The viral type II topoisomerase encoded by the African swine fever virus (ASFV) is critical for viral replication and infection, thus representing an attractive target for antiviral drug development. Type II topoisomerases can relax supercoiled DNA by a concerted strand-passage mechanism in which the enzyme first cleaves one DNA duplex (G-segment) and then guides the second DNA duplex (T-segment) to pass through the transient breaks. ASFV P1192R contains two conserved domains, namely, an N-terminal ATPase domain and a central DNA cleavage core followed by a coiled-coil arm, but lacks the nonconserved C-terminal domain (CTD) with modulating activities reported in human topo II. Similar to previously reported topo II structures of yeast and human, P1192R assembles into a large homodimer mediated by two interfaces.

Interestingly, 3D classification revealed two distinct classes with almost even particle populations, generating high-resolution reconstructions with C2 symmetry imposed at an overall resolution of 3.16 Å and 3.13 Å, respectively. One state has a closed conformation in the C-terminal dimer interface, and the other one appears open. In our study, two distinct P1192R dimeric states were observed simultaneously in the cryo-EM samples, with their DNA-gate closed, whereas their C-gate is closed and open, respectively. In the open state structure, the interface of coiled-coil arms separates by ~17 Å, comparable with reported C-gate opening structures, thereby displaying an opening C-gate conformation. It shows that the conformations of the DNA cleave core for the two P1192R dimers are nearly identical, with a root-mean-square deviation (RMSD) value of 1.25 Å for all Cα. Compared with the yeast topo II, P1192R contains an additional pair of E817-R1046 salt bridge, which is retained in the closed state while disrupted in the open state. Comparison of the open states of P1192R and yeast topo II showed that the distance of the C-gate gap is nearly equal; however, the coiled-coil arm displays a 15° rotation between the two structures. In addition, we found that the open state of the P1192R, yeast, and human topo II shared a similar opening distance (~17 Å) of the C-gate, while differing in the conformation of the coiled-coil arm. Since no DNA substrates are present in the cryo-EM samples, we consider that the C-gate could adopt both closed and open conformations prior to reaction, and its status might be self-regulated through inter-domain interactions. The N-terminal ATPase domain comprising amino acids 1–414 was invisible in both states, probably owing to its flexible connection with the other part of P1192R.

>MEAFEISDFKEHAKKKSMWAGALNKVTISGLMGVFTEDEDLMALPIHRDHCPALLKIFDEIIVNATDHERACHNKTKKVTYIKISFDKGVFSCENDGPGIPIAKHEQASLIAKRDVYVPEVASCHFLAGTNINKAKDCIKGGTNGVGLKLAMVHSQWAILTTADGAQKYVQHINQRLDIIEPPTITPSREMFTRIELMPVYQELGYAEPLSETEQADLSAWIYLRACQCAAYVGKGTTIYYNDKPCRTGSVMALAKMYTLLSAPNSTIHTATIKADAKPYSLHPLQVAAVVSPKFKKFEHVSVINGVNCVKGEHVTFLKKTINEMVVKKFQQTIKDKNRKTTLRDSCSNIFIVIVGSIPGIEWTGQRKDELSIAENVFKTHYSIPSSFLTSMTKSIVDILLQSISKKDNHKQVDVDKYTRARNAGGKRAQDCMLLAAEGDSALSLLRTGLTLGKSNPSGPSFDFCGMISLGGVIMNACKKVTNITTDSGETIMVRNEQLTNNKVLQGIVQVLGLDFNCHYKTQEERAKLRYGCIVACVDQDLDGCGKILGLLLAYFHLFWPQLIIHGFVKRLLTPLIRVYEKGKTMPVEFYYEQEFDAWAKKQTSLANHTVKYYKGLAAHDTHEVKSMFKHFDNMVYTFTLDDSAKELFHIYFGGESELRKRELCTGVVPLTETQTQSIHSVRRIPCSLHLQVDTKAYKLDAIERQIPNFLDGMTRARRKILAGGVKCFASNNRERKVFQFGGYVADHMFYHHGDMSLNTSIIKAAQYYPGSSHLYPVFIGIGSFGSRHLGGKDAGSPRYISVQLASEFIKTMFPAEDSWLLPYVFEDGQRAEPEYYVPVLPLAIMEYGANPSEGWKYTTWARQLEDILALVRAYVDKDNPKHELLHYAIKHKITILPLRPSNYNFKGHLKRFGQYYYSYGTYVISEQRNIITITELPLRVPTVAYIESIKKSSNRMTFIEEIIDYSSSETIEILVKLKPNSLNRIVEEFKETEEQDSIENFLRLRNCLHSHLNFVKPKGGIIEFNTYYEILYAWLPYRRELYQKRLMREHAVLKLRIIMETAIVRYINESAELNLSHYEDEKEASRILSEHGFPPLNHTLIISPEFASIEELNQKALQGCYTYILSLQARELLIAAKTRRVEKIKKMQARLDKVEQLLQESPFPGASVWLEEIDAVEKAIIKGRNTQWKFH[2x]>[2x]MNYFVGNSLGVNLTGIEKAIINRLNLFKEMGRPAQCVFLSWNRYLYRNAQNYITSSDYINMYDFFQEATYLERNEPFDWLSYWTDECHYTLKHVENSHDFRIYDQERFLMYAHFQDPKYRILDYVNHFDSQRRKVKRDFYDVRGFLSCSRILVDKQQTLCEF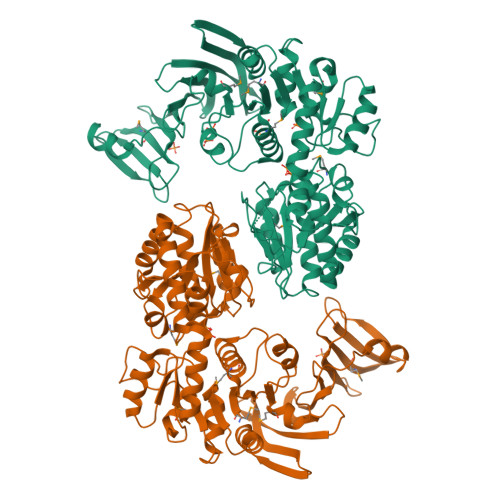FYNPEGDTKLEKYFSYKDGKPEVQKIIVYYANKQYFFNNETELGAFFIKQLYQHGDLFFSDRNVYTAPIFNLTPESIPVVAVLHSTHIKNIDALDSSPFKNVYKAMFENLSRYRAIIVSTEQQKLDVEKRINHTIPVVNIPVGYSETIDTPVQTLDQRSVKLISVARYSPEKQLHQQIELIKRLVSYVPKIELHMYGFGSESKKLNELIQKYGLENHVYLRGFLSNLDQEYSDAYLSLITSNMEGFSLALLESLAHGVPVISYDIKYGPNELITSDFNGYLITKNDEDALFDKVKYVIDHPEVQQRLSKGSLAKAQQYSKASLIKQWDQFVRLILEHHHHHH(2S)-2-(3-{[AMINO(IMINO)METHYL]AMINO}PHENYL)-3-[(R)-[(1R)-1-({N-[(BENZYLOXY)CARBONYL]-L-PHENYLALANYL}AMINO)-2-METHYLPROPYL](HYDROXY)PHOSPHORYL]PROPANOIC ACID | C31 H38 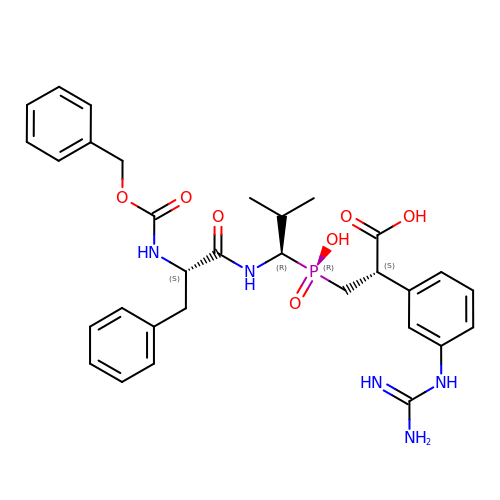N5 O7 P | SYQCJJZICSZGRU-UNCTUWKVSA-N> KAQTTSHELTIPNDLIGCIIGRQGAKINEIRQMS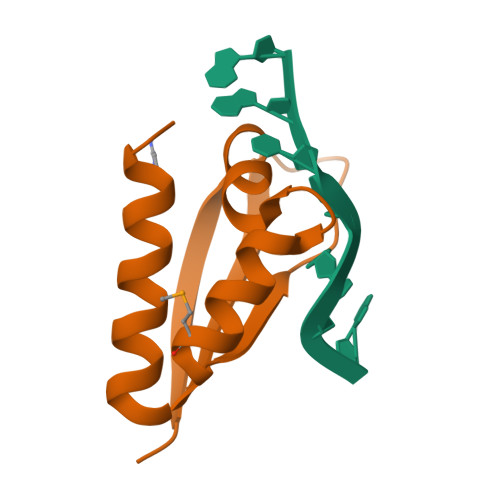GAQIKIANPVEGSTDRQVTITGSAASISLAQYLINVRLSSET>[2x]GAMALPSGSDPAFSQPKSVLDAGLTCQGASPSSVSKPILLVPGTGTTGPQSFDSNWIPLSAQLGYTPCWISPPPFMLNDTQVNTEYMVNAITTLYAGSGNNKLPVLTVCQGGLVAQWGLTFFPSIRSKVDRLMAFAPDYKGTVLAGPLDALAGSAPSVWQQTTGSALTTALRNAGGLTQIVPTTNLYSATDEIVQPQVSNSPLDSSYLFNGKNVQ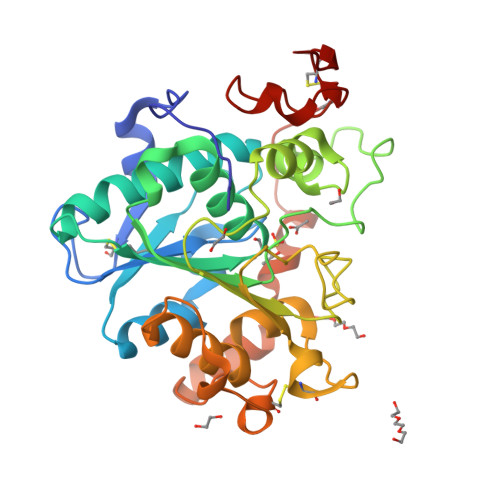AQAVCGPLFVIDHAGSLTSQFSYVVGRSALRSTTGQARSADYGITDCNPLPANDLTPEQKVAAAALLAPYYAAIVAGPKQNCEPDLMPYARPFAVGKRTCSGIVTP> CAUCCGGUAUCCCAAGACAUCUUCGGGUGGGUUGGGAAGUAUCAUGGCUAAUCACCAUGAUGCAAUCGGGUUGAACACUUAAUUGGGUUAAAACGGUGGGGGACGAUCCCGUAACAUCCGUCCUAACGGCGA;> G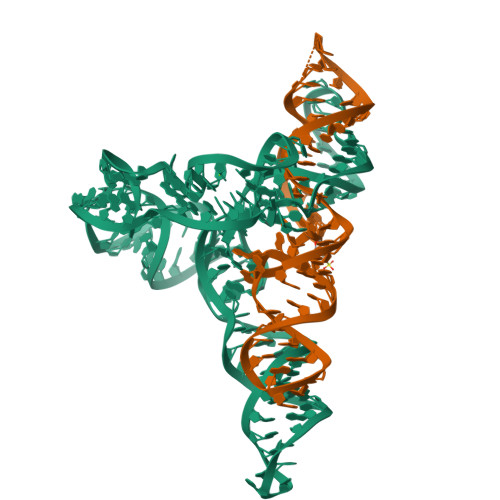ACUGCACGGCCCUGCCUCAGGUGUGUUCAAUGAACAGUCGUUCCGAAAGGAAG>[6x]MDFYYLPGS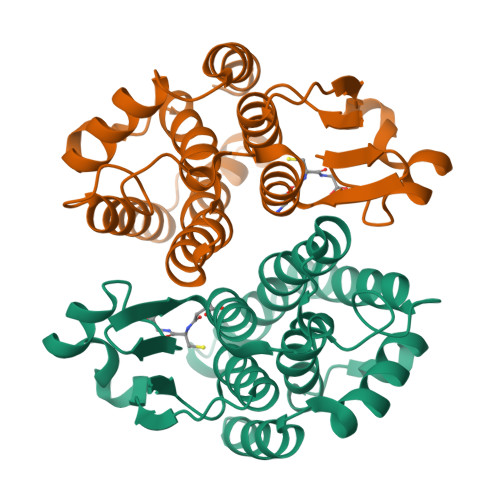APCRAVQMTAAAVGVELNLKLTNLMAGEHMKPEFLKINPQHCIPTLVDNGFALWESRAICTYLAEKYGKDDKLYPKDPQKRAVVNQRLYFDMGTLYQRFADYYYPQIFAKQPANAENEKKMKDAVDFLNTFLDGHKYVAGDSLTIADLTVLATVSTYDVAGFELAKYPHVAAWYERTRKEAPGAAINEAGIEEFRKYFEK5-[4-[(2~{R},3~{S},4~{S},5~{S},6~{R})-6-(hydroxymethyl)-3,4,5-tris(oxidanyl)oxan-2-yl]oxy-3-methyl-phenyl]-~{N}1,~{N}3-dimethyl-benzene-1,3-dicarboxamide 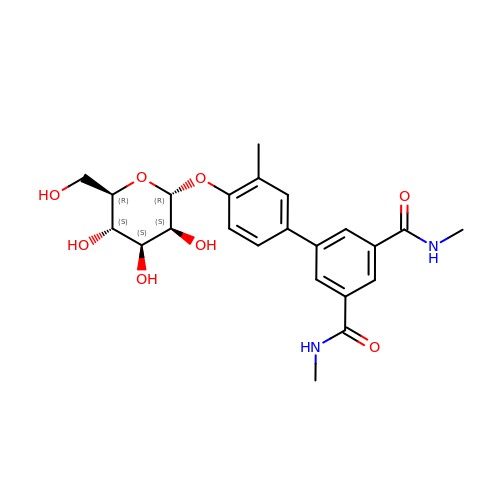| C23 H28 N2 O8 | CPNXCPWXQQMNFG-WCZGSDDISA-N>MATNFFIQPITEEAEAYYPPSVITNKRKDLGVDVYCCSDLVLQPGLNIVRLHIKVACEHMGKKCGFKIMARSSMCTHERLLILANGIGLIDPGYVGELMLKIINLGDTPVQIWAKECLVQLVAQGDHVPDHINILKRNQIFPLFAPTPRGEGRFGSTGEAGIMRTHHHHHH[3x]

ASFV encodes a dUTP nucleotidohydrolase (dUTPase) (dUTP pyrophosphatase [Dut]; EC 3.6.1.23), called E165R. The enzyme degrades dUTP in the cytoplasm and thus minimizes misincorporation of uracil into viral DNA, which plays an essential role in maintaining the fidelity of genome replication. It is indispensable for reproductive infection of ASFV in swine macrophages, the natural host cell for the virus. We show that E165R is a homotrimer and can specifically hydrolyze dUTP.

However, we obtained the crystal structure of E165R-dUMP complex rather than E165R-dUTP complex at a resolution of 1.70 Å, with Rwork and Rfree values of 18.8% and 21.5%, respectively. This result further confirmed that E165R has a pyrophosphatase activity that degrades dUTP into dUMP and pyrophosphoric acid. Each of the three dUMP binds to the interface of two protomers of the E165R trimer. dUMP interacts with N85, G88, L89, I90, D91, Y94, and M99 of one E165R protomer and R71, S72, and Q120 of another protomer. Among these interactions, N85, D91, and M99 from one protomer form hydrogen bonds with the deoxyuridine part of dUMP, while S72 and Q120 from the other protomer form hydrogen bonds with the phosphate group of dUMP. All three E165R subunits in the crystal structure of E165R-dUMP complex contain 1 to 144 residues of the total 165 residues of E165R, and the 21 residues at the C terminus are invisible due to poor electronic density. The secondary structure of the E165R protein in the E165R-dUMP complex is very similar to that of apo-E165R, except that the C-terminal 310 helix in apo-E165R is missing in the E165R-dUMP complex. There are certain anticlockwise rotations of each E165R-dUMP subunit relative to their corresponding subunits in apo-E165R. In contrast, these values become 127.0 Å2 and 62.2 Å3, respectively, for the binding pockets in the E165R-dUMP complex. However, we did not found any magnesium ion, free pyrophosphoric, or phosphoric acid groups in the binding pocket of the E165R-dUMP complex, just like in other dUTPase-dUMP complexes.> MGKDQLDFSHFDKAFENKYDIVAPEFGDLHQKRAEFIAKNQGTYRPVPLVPNNIKGLIPKTCRLPATRNWYRRTSSF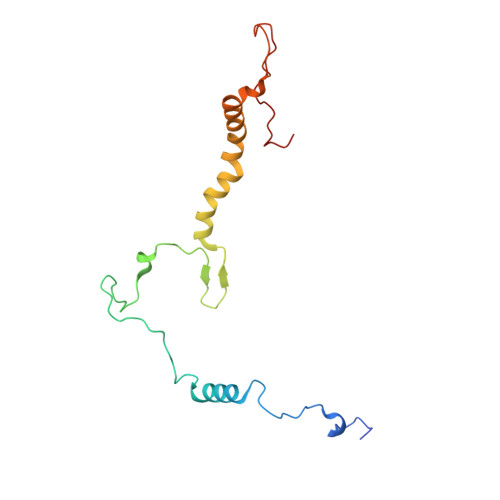ERNGFFNIHTPVLNTKMIPWLLFIVLTWGWSSFQIGGYNYERFDDNGERRNTLYWKLSPVEFPQSKLWNRPS WsaF is the first rhamnosyltransferase to be structurally and biochemically characterised. WsaE is a multifunctional enzyme forming both an α-1,2- and the α-1,3-linkage; WsaF is a β-1,2-rhamnosyltransferase. Both enzymes utilise dTDP-β-l-rhamnose (dTDP-β-l-Rha) as the donor molecule. In the CAZy database, WsaF is annotated to GT4 family, which is the largest retaining GT-B fold family with currently 11,446 entries.

The crystal structure of WsaF was determined using single-wavelength anomalous diffraction of selenomethionine (SeMet)-labeled WsaF crystals at 2.28 Å resolution. The N-terminal domain comprises residues F26-F222, and the C-terminal domain is formed from residues T228-N381. The two domains are connected by the loop Q223-N227. The C-terminal α-helix S390-L413 crosses between the two domains and forms part of the N-terminal domain. The N-terminal domain has an eight-stranded β-sheet that is bounded by six α-helices. The C-terminal domain has a seven-stranded β-sheet that is flanked by five α-helices. Three regions of the structure have poor or no electron density, indicating conformational flexibility: the N-terminal M1-N25, the loop between β1 and α1 in the N-terminus (Q58-G63), and the loop that connects the C-terminal α-helix to the rest of the protein (N382-E389). In the crystal, two WsaF monomers form a dimer related by 2-fold symmetry. The dimer buries 1900 Å2 of solvent-accessible surface per monomer, and the statistical score provided by PISA indicates a dimer, which is also stable in solution. The conformation of K302 is disordered in the native structure.

>[2x]MLQKLIQILRRNEYVKNVYKNTVSNFIETSIPEITPFNARTSSIKGKRLNLLVPSINQEHMFGGISTALKLFEQFDNKKFKKRIILTDATPNPKDLQSFKSFKYVMPEEDKDFALQIVPFNDRYNRTIPVAKHDIFIATAWWTAYAAQRIVSWQSDTYGIPPNKILYIIQDFEPGFYQWSSQYVLAESTYKYRGPQIAVFNSELLKQYFNNKGYNFTDEYFFQPKINTTLKNYINDKRQKEKIILVYGRPSVKRNAFTLIVEALKIFVQKYDRSNEWKIISVGEKHKDIALGKGIHLNSLGKLTLEDYADLLKRSSIGISLMISPHPSYPPLEMAHFGLRVITNKYENKDLSNWHSNIVSLEQLNPENIAETLVELCMSFNNRDVDKKESSNMMFYINEFNEFSFIKEIEEKL> SNAVTYPLPTDGSRLVGQNQVITIPDDNKQPLEYFAAKYQMGLSNMLEANPGVDTYLPKGGSVLNIPQQLILPDTVHEGIIINSAEMRLYYYPKGTNTVIVLPIGIGQLGKDTPINWTTKVERKKAGPTWTPTAKMHAEYAAAGNPLPAVVPAGPDNPMGLYALYIGRLYAIHGTNANFGIGLRVSHGCVRLRNDDIKFLFENVPVGTRVQFIDEPVKATTEPDGSRYIEVH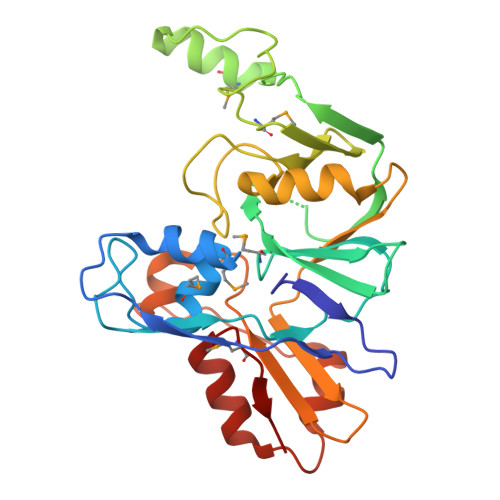NPLSTTEAQFQGGEIVPITLTQPVQAVTSQSDVDQNVVEQAIQNRSGMPVRLN> MKLTPKELDKLMLHYAGELAKKRKEKGIKLNYVEAVALISAHIMEEARAGKKTAAELMQEGRTLLKPDDVMDGVASMIHEVGIEAMFPDGTKLVTVHTPIEANGKLVPGELFLKNEDITINEGKKAVSVKVKNVGDRPVQIGSHFHFFEVNRCLDFDREKTFGKRLDIAAGTAVRFEPGEEKSVELIDIGGNRRIFGFNALVDRQADNESKKIALHRAKERGF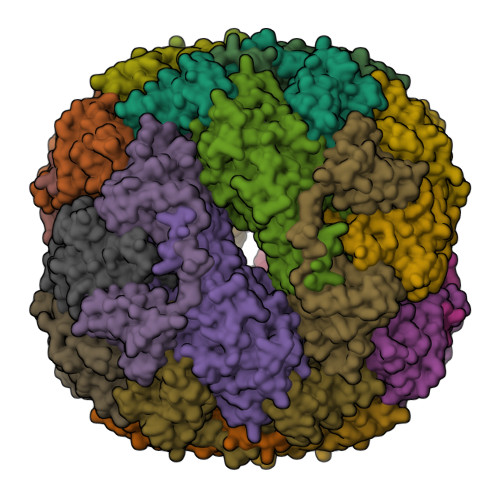HGAKSDDNYVKTIKE;> MKKISRKEYVSMYGPTTGDKVRLGDTDLIAEVEHDYTIYGEELKFGGGKTLREGMSQSNNPSKEELDLIITNALIVDYTGIYKADIGIKDGKIAGIGKGGNKDMQDGVKNNLSVGPATEALAGEGLIVTAGGIDTHIHFISPQQIPTAFASGVTTMIGGGTGPADGTNATTITPGRRNLKWMLRAAEEYSMNLGFLAKGNASNDASLADQIEAGAIGFKIHEDWGTTPSAINHALDVADKYDVQVAIHTDTLNEAGCVEDTMAAIAGRTMHTFHTEGAGGGHAPDIIKVAGEHNILPASTNPTIPFTVNTEAEHMDMLMVCHHLDKSIKEDVQFADSRIRPQTIAAEDTLHDMGAFSITSSDSQAMGRVGEVITRTWQTADKNKKEFGRLKEEKGDNDNFRIKRYLSKYTINPAIAHGISEYVGSVEVGKVADLVLWSPAFFGVKPNMIIKGGFIALSQMGDANASIPTPQPVYYREMFAHHGKAKYDANITFVSQAAYDKGIKEELGLERQVLPVKNCRNVTKKDMQFNNTTAHIEVNPETYHVFVDGKEVTSKPANKVSLAQLFSIF> GSKLPP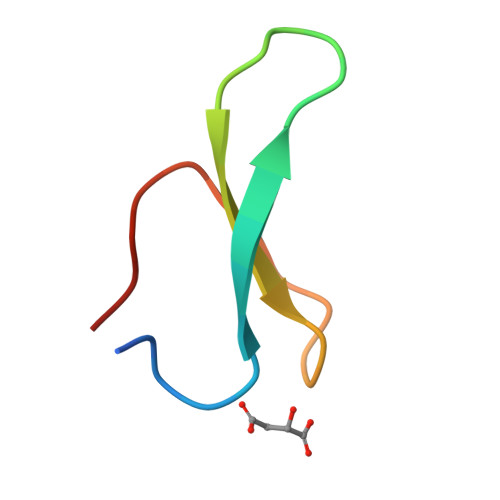GWEKRMSRSSGRVYYFNHITNASQWERPSG>MKKALICIDYTNDFAAENGALTCGEPARQIEDTIVSLTQAFIENGDYVVFAVDSHDA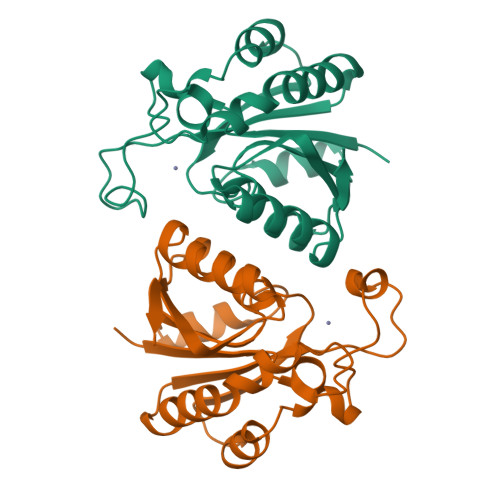DDDFHPETRLFPPHNINGTEGKELYGRLSPLYEKHKHAKNVNYMEKTRYSAFAGTDLELKLRERQIAELHLAGLCTDICVLHTAVDAYNKGFQIVIHQNAVASFNPEGHEWALSHFKNSIGAQVAE[2x]> MGQSEPIVLVIFTNKDNKSDKPNDKLISETAKSVMKEFAAGSKNAAKELNDLEKKYNAHIGVYALDTKSGKEVKFNSDKRFAYASTSKAINSAILLEQVPYNKLNKKVHINKDDIVAYSPILEKYVGKDITLKALIEASMTYSDNTANNKIIKEIGGIKKVKQRLKELGDKVTNPV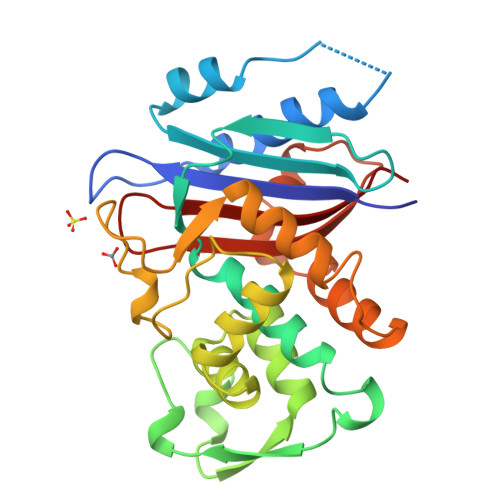RYEIELNYYSPKSKKDTSTPAAFGKTLNKLIANGKLSKENKKFLLDLMLNNKSGDTLIKDGVPKDYKVADKSGQAITYASRNDVAFVYPK1-({7-[(2R)-5-chloro-2-(piperazine-1-carbonyl)-2,3-dihydro-1-benzofuran-7-yl]thieno[3,2-b]pyridin-2-yl}methyl)-1H-pyrrole-2,5-dione 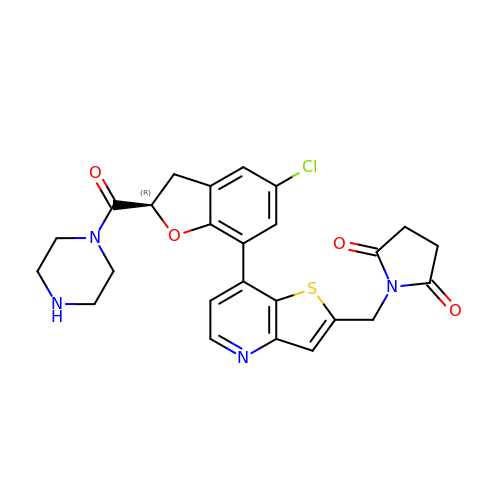| C25 H23 Cl N4 O4 S | HDYYKIHPDVFOOZ-HXUWFJFHSA-N~{N}-[4-[(3~{R})-piperidin-3-yl]oxyphenyl]-1~{H}-pyrrolo[2,3-b]pyridin-4-amine | C18 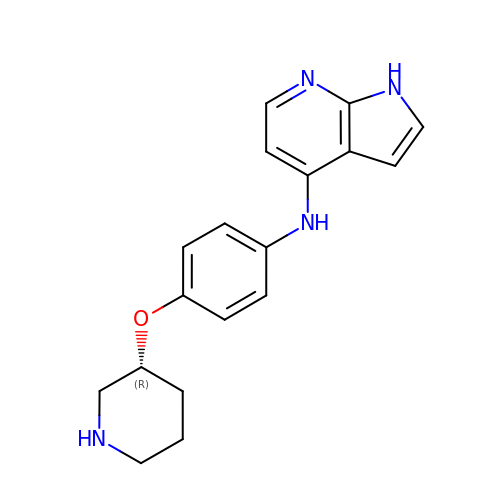H20 N4 O | IYFCFYWXRIVCTH-OAHLLOKOSA-N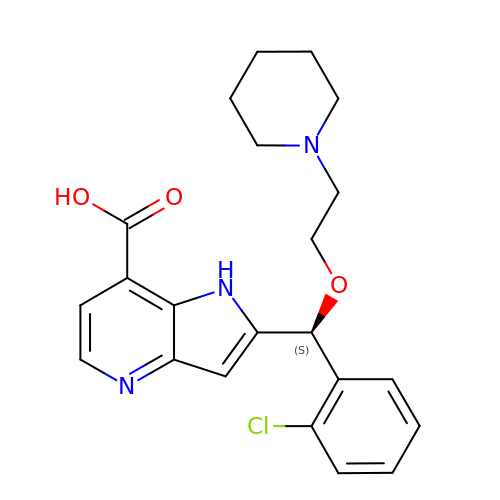2-{(S)-(2-chlorophenyl)[2-(piperidin-1-yl)ethoxy]methyl}-1H-pyrrolo[3,2-b]pyridine-7-carboxylic acid | C22 H24 Cl N3 O3 | AWPYWZMMJZGPOX-NRFANRHFSA-N> GPGSFKERRPFHERQKDVEEIRSQQPNKVPVIIERFDGERSLPLMDRCKFLVPEHITVAELMSIVRRRL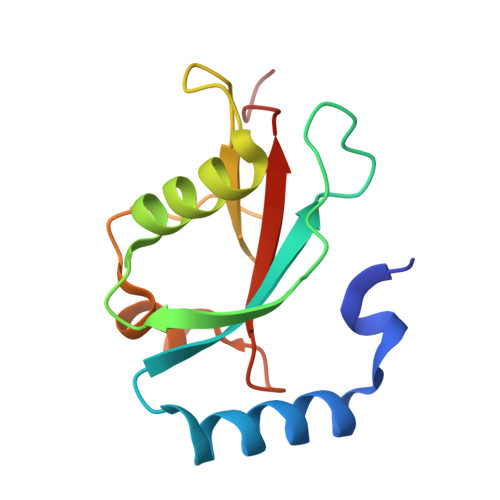QLHPQQAFFLLVNERSMVSNSMSMSNLYSQERDPDGFVYMVYTSQPAFG>GFGCNGPWSEDDMKCHNHCKSIKGYKGGYCAKGGFLCKCY[42x]

Plectasin consists of 40 amino acids and shows well-defined secondary structural elements in form of an α-helix (M13-S21) and an antiparallel β-sheet (G28-A31; V36-C39). The structure of plectasin is stabilized by three disulfide bridges (C4-C30; C15-C37; C19-C39), which is typical for this type of defensins and leads to high conformational stability. Plectasin contains a cysteine-stabilised α-helix-β-sheet structure, which remains intact upon fibril formation. We have determined the structure, kinetics, and functionality associated with the pH-responsive self-assembly of the enhanced plectasin variant PPI42 into helical protein fibrils.

We were able to determine the structure of the plectasin fibril at an overall resolution of 1.97 Å (local resolution varies between 1.9 and 3.0 Å) using cryo-EM, which is one of the highest resolutions hitherto achieved for a protein fibril in cryo-EM and allowed an unambiguous structure determination. The structure consists of two coiling protofilaments, which form a right-handed superstructure (mature fibril). Each protofilament has an axial (C2) and a helical symmetry (axial rise z = 25.20 Å and a helical twist phi = 15.75°). The repeating or asymmetric unit (au) for each protofilament is composed of seven monomers. They are arranged in a near-helical way by forming a pseudo-right-handed helix with an average axial rise of 3.75 ± 0.15 Å and an average twist of 156.48 ± 2.25° between two consecutive monomers. The PPI42 protofilament is stabilized by a hydrophobic core in the centre (red spheres) and hydrophobic interfaces between the monomers (black spheres). Even though the local resolution is lower in that region (~2.5 Å), we could conclude that the negatively charged sidechains of (E10) and (D11) appear to play an essential role in the arrangement of PPI42 in the protofilament by forming a network of salt bridges to different lysines. The assembly of the two protofilaments into the superstructure is favoured by the interaction of the loop between α-helix and β-sheet of monomer 1 and 3 in each asymmetric unit with the two symmetric monomers in the other protofilament. The (G24)1 and (K23)1 backbone form three hydrogen bonds with the (K23)3 sidechain and backbone and (S21)3 backbone which stabilize the mature fibril. The interface between the two protofilaments was calculated to be 722 Å2 per asymmetric unit, which corresponds to a small interface area for protein complexes.>MARKFFVGGNFKMNGSLESMKTIIEGLNTTKLNVGDVETVIFPQNMYLITTRQQVKKDIGVGAQNVFDKKNGAYTGENSAQSLIDAGITYTLTGHSERRTIFKESDEFVADKTKFALEQGLTVVACIGETLAEREANTINVVVRQLNAIADKVQ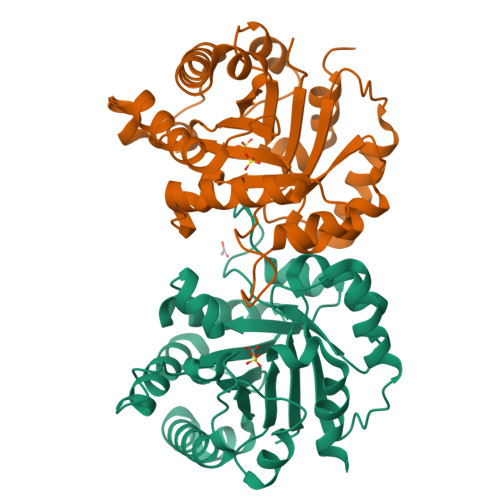NWSKIVIAYEPVWAIGTGKTATPEQAQEVHAEIRKWATNKLGASVAEGLRVIYGGSVNGGNCKEFLKFHDIDGFLVGGASLKPEFHNIVNVHSL[4x]>[8x]A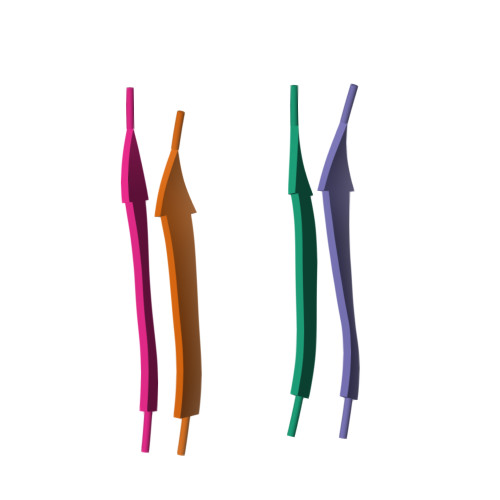IIGLM>MVTKTITEQRAEVRIFAGNDPAHTATGSSGISSPTPALTPLMLDEATGKLVVWDGQKAGSAVGILVLPLEGTETALTYYKSGTFATEAI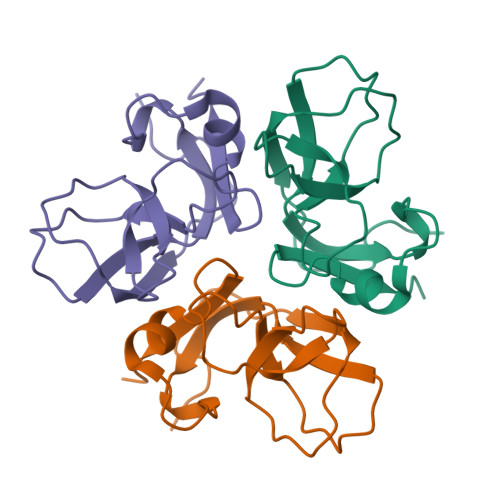HWPESVDEHKKANAFAGSALSHAALP[3x]BK polyomavirus (BKPyV) is a small, non-enveloped, double-stranded DNA virus with an icosahedral capsid formed by 72 capsomers, where a capsomer is an association of a pentamer of the VP1 protein linked internally to a single copy of either the VP2 or the VP3 proteins. BK polyomavirus (BKPyV) is an opportunistic pathogen that uses the b-series gangliosides GD1b and GT1b as entry receptors. Viruses sampled sequentially from these patients accumulated multiple mutations in the BC loop region of the VP1 protein, which is involved in the direct interaction of the virus with sialic acids. All variant VP1 pentamer structures were globally similar to the WT VP1 pentamer with a doughnut-shaped ring composed of a central pore surrounded by five VP1 monomers in 5-fold symmetry.

The E73Q pentamer structure was almost identical to that of the WT (RMSD in the BC loop region, from amino acids 68–76, of 0.5 Å), whereas the E73A mutant presenting an alanine in the same position showed some structural changes. Specifically, the S-shaped curve of the backbone structure between amino acids 72 to 75 of the BC2 loop appeared to be flipped over in two monomers out of the five. We therefore refer to this conformational change as “BC loop flipping. However, two monomers retained the WT loop conformation, while the last monomer seemed to have a state where both conformations are superimposed, leading to two different RMSD values for the BC loop of the E73A crystal (1.2 Å for WT loop conformation and 1.5 Å for the alternative conformation). Thus, the mutation to alanine induces a more flexible conformation for the loop compared with the WT and the E73Q single mutant. Variants E73A, E73Q, and VQQ all showed broader ganglioside binding, indicating that negative charge at residue 73 may restrict WT BKPyV VP1 binding to b-series gangliosides, and that removing this charge is sufficient to allow binding to a-series gangliosides. In 293TT cells, the E73Q variant was as infectious as the WT, while E73A and N-Q variants showed 3-fold lower infectivity, and VQQ variant was barely infectious. In RS cells, the ability to use GD1a as an entry receptor results in the strongly increased infectivity of the E73Q variant, whereas for E73A and VQQ, enhanced ganglioside binding was balanced by a loss of infectivity due to BC loop flipping, leading to near-WT infectivity for both variants.

>[5x]GGVEVLEVKTGVDAITEVECFLNPEMGDPDENLRGFSLKLSAANDFSSDSPERKMLPCYSTARIPLPNLNEDLTSGNLLMWEAVTVQTEVIGITSMLNLHAGSQKVHEHGGGKPIQGSNFHFFAVGGEPLEMQGVLMNYRSKYPDGTITPKNPTAQSQVMNTDHKAYLDKNNAYPVECWVPDPSRNENARYFGTFTGGENVPPVLHVTNTATTVLLDEQGVGPLCKADSLYVSAADICGLFTNSSGTQQWRGLARYFKIRLRKRSVKNPYP5'-O-[(R)-hydroxy(phosphonoamino)phosphoryl]adenosine | C10 H16 N6 O9 P2 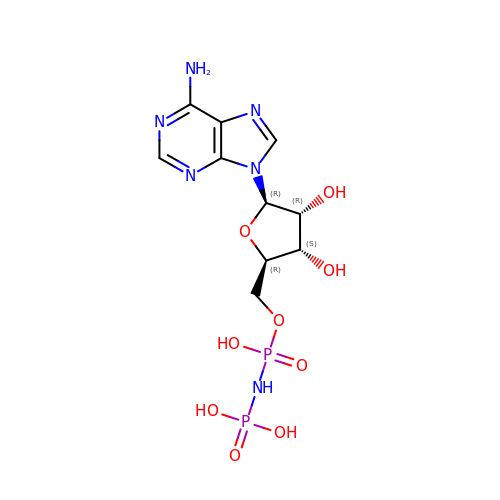| FJNYKURUYWTJIG-KQYNXXCUSA-N>[2x]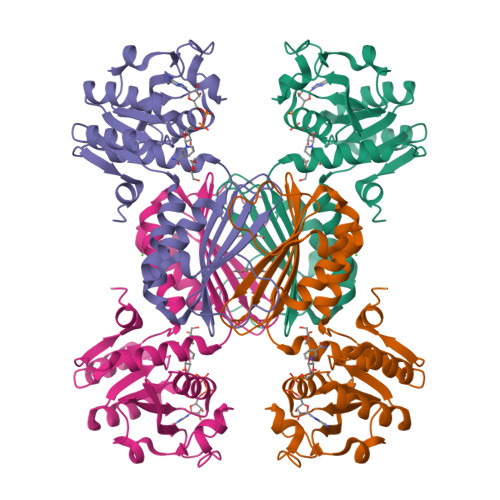MAHHHHHHMRRIAVVGAAGRMGKNLIEAVQQTGGAAGLTAAVDRPDSTLVGADAGELAGLGRIGVPLSGDLGKVCEEFDVLIDFTHPSVTLKNIEQCRKARRAMVIGTTGFSADEKLLLAEAAKDIPIVFAANFSVGVNLCLKLLDTAARVLGDEVDIEIIEAHHRHKVDAPSGTALRMGEVVAQALGRDLQEVAVYGREGQTGARARETIGFATVRAGDVVGDHTVLFAAEGERVEITHKASSRMTFARGAVRAALWLEGKENGLYDMQDVLGLR>[2x]QEDVTVKSVTLITKVFPEGEKVCAVVIEYPVEIDGQKLSPDQFSVKVKTGDTYSSRTITKVYANNSGGLSFSIFNNRGKYVVLELSTEDLHSNTIVFGPNFLNTRMKLDYIVSQLVPIFDVDGNEV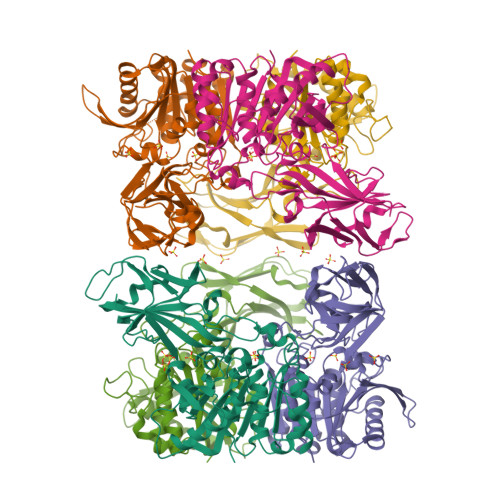EPFTSKQTDEKHLIIDDFLAFTFKDPETGVEIPYRLFVPKDVNPDRKYPLVVFLHGAGERGTDNYLQVAGNRGAVVWAQPRYQVVHPCFVLAPQCPPNSSWSTLFTDRENPFNPEKPLLAVIKIIRKLLDEYNIDENRIYITGLSMGGYGTWTAIMEFPELFAAAIPICGGGDVSKVERIKDIPIWVFHAEDDPVVPVENSRVLVKKLAEIGGKVRYTEYEKGFMEKHGWDPHGSWIPTYENQEAIEWLFEQSR>MSTVGTGKLTRAQRRAAARKNKRNTRVVQPVIVEPIASGQGKAIKAWTGYSVSKWTASCAAAEAKVTSAITISLPNELSSERNKQLKVGRVLLWLGLLPSVSGTVKSCVTETQTTAAASFQVALAVADNSKDVVAAMYPEAFKGITLEQLTADLTIYLYSSAALTEGDVIVHLEVEHVRPTFDDSFTPVY[3x]

Cowpea chlorotic mottle virus is an icosahedrally symmetric plant virus in the Bromoviridae family that infects cowpea plants (Vigna unguiculata). The 180 identical capsid proteins are arranged in 12 pentamers and 20 hexamers. The asymmetric unit (highlighted) contains three subunits A, B, and C (magenta, green, and blue, respectively). CCMV is thought to achieve this by detecting a change in its chemical environment upon entering the host cell, which causes its capsid to swell, increasing in diameter by about 10%2.

Cryo samples of extended CCMV at pH 7.6 (containing no divalent ions) are prepared in the presence of a photoacid (NPE-caged-proton). The sample was plunge-frozen at pH 7.6, after which the pH was lowered to 4.5 by releasing the photoacid. The capsid has a diameter of 32 nm, with the disordered RNA in its interior not resolved. The reconstruction is indistinguishable from one obtained without first lowering the pH. This confirms that the vitreous ice matrix has prevented the particles from contracting, even though the negatively charged residues whose repulsion keeps the capsid inflated are likely protonated due to the high proton conductivity of vitreous ice. Once the calcium ions are no longer present to compensate these negative charges, electrostatic repulsion causes the capsid to expand. We then dock atomic models of the extended configuration into slices 1–12 (extended and partially contracted particles) and of the contracted configuration into slices 25–30 (fully contracted particles), from which we determine the motions of the capsid proteins. However, when we rapidly melt the sample with a laser beam (532 nm), the particles begin to contract as soon as the sample is liquid. When we prepare CCMV in its extended state and lower the pH to 4.5, melting and revitrification of the sample allows the particles to partially contract.> AGTDNPT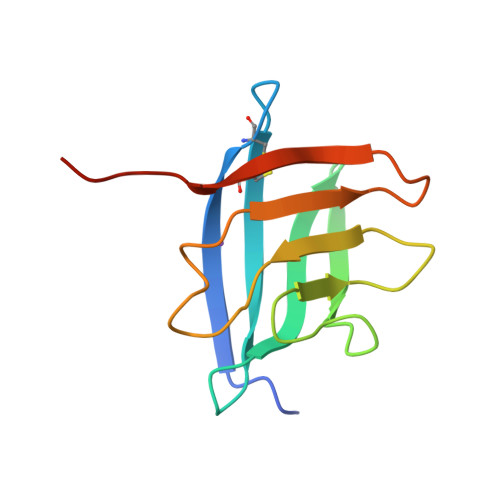VAKKTVSYVCQQGKKVKVTYGFNKQGLTTYASAVINGKRVQMPINLDKSDNMDTFYGKEGGYVLSTGAMDSKSYRKQPIMITAPDNQIVFKDCSPRLEHHHHHH> MKMKMKLASFGLAAGLAAQVFLPYNALASTEHVTWNQQFQTPQFISGDLLKVNGTSPEELVYQYVEKNENKFKFHENAKDTLQLKEKKNDNLGFTFMRFQQTYKGIPVFGAVVTSHVKDGTLTALSGTLIPNLDTKGSLKSGKKLSEKQARDIAEKDLVANVTKEVPEYEQGKDTEFVVYVNGDEASLAYVVNLNFLTPEPGNWLYIIDAVDGKILNKFNQLDAAKPGDVKSITGTSTVGVGRGVLGDQKNINTTYSTYYYLQDNTRGNGIFTYDAKYRTTLPGSLWADADNQFFASYDAPAVDAHYYAGVTYDYYKNVHNRLSYDGNNAAIRSSVHYSQGYNNAFWNGSQMVYGDGDGQTFIPLSGGIDVVAHELTHAVTDYTAGLIYQNESGAINEAISDIFGTLVEFYANKNPDWEIGEDVYTPGISGDSLRSMSDPAKYGDPDHYSKRYTGTQDNGGVHINSGIINKAAYLISQGGTHYGVSVVGIGRDKLGKIFYRALTQYLTPTSNFSQLRAAAVQSATDLYGSTSQEVASVKQAFDAVGVK

Here, an automated procedure is described to identify the positions of many cryocooled crystals mounted on the same sample holder, to rapidly predict and rank their relative diffraction strengths and to collect partial X-ray diffraction data sets from as many of the crystals as desired. Subsequent hierarchical cluster analysis then allows the best combination of partial data sets, optimizing the quality of the final data set obtained. To demonstrate the general applicability of the workflow described here, we have applied it to various systems and scenarios in which many crystals of the same type are mounted on the same cryocooled sample holder. In all of the cases presented our workflow has yielded data sets that are fit for purpose.

In order to demonstrate the possibilities of the workflow presented here to produce data suitable for experimental phasing techniques that exploit anomalous scattering, two different systems were investigated. The first of these, thermolysin, contains one catalytic Zn2+ ion and three Ca2+ ions per protein chain (316 residues), producing a theoretical anomalous diffraction ratio (〈ΔF/F〉) of ∼2% for data collected at the peak of the Zn K absorption edge. Bacillus thermoproteolyticus thermolysin (Sigma–Aldrich catalogue No. T0331) was dissolved to 100 mg ml−1 in 45% DMSO, 0.05 M MES pH 6.0. The reservoir contained 35% saturated ammonium sulfate, whereas the drops were composed of the protein solution and a solution consisting of 0.05 M MES pH 6.0, 1 M NaCl, 45% DMSO in a 1:1 ratio. Rod-shaped crystals of between 40 × 40 × 150 and 40 × 40 × 300 µm in size were quick-soaked in 6 M trimethylamine N-oxide (TMAO; Mueller-Dieckmann et al., 2011) for cryoprotection before mounting on a sample support. Diffraction data were collected using an X-ray beam of 10 µm in diameter with a flux of 4.0 × 1010 photons s−1 at the peak of the Zn K absorption edge (λ = 1.256 Å) on beamline ID23-1 of the ESRF. Our experiments with crystals of thermolysin reveal other features of the developed pipeline. The workflow thus ensures that partial data sets are collected from only well diffracting areas of any given crystal. The collection of data of sufficiently high quality for the structure solution of both systems is thus clearly challenging, even from single crystals. Nevertheless, as can be seen in Figs. 6 and 7, for both systems our multi-crystal workflow clearly yields diffraction data of sufficient quality for structure solution.>GAAAGVAAWLPFARAAAIGWMPVANCPMPLAPADKNKRQDELIVLNVSGRRFQTWRTTLERYPDTLLGSTEKEFFFNEDTKEYFFDRDPEVFRCVLNFYRTGKLHYPRYECISAYDDELAFYGILPEIIGDCCYEEYKDRKREN[8x];>[8x]EGLEQLEAQTNFTKRELQVLYRGFKNECPSGVVNEDTFKQIYAQFFPHGDASTYAHYLFNAFDTTQTGSVKFEDFVTALSILLRGTVHEKLRWTFNLYDINKDGYINKEEMMDIVKAIYDMMGAYTYPVLAEDTPRQHVDVFFQKMDKNKDGIVTLDEFLESCQE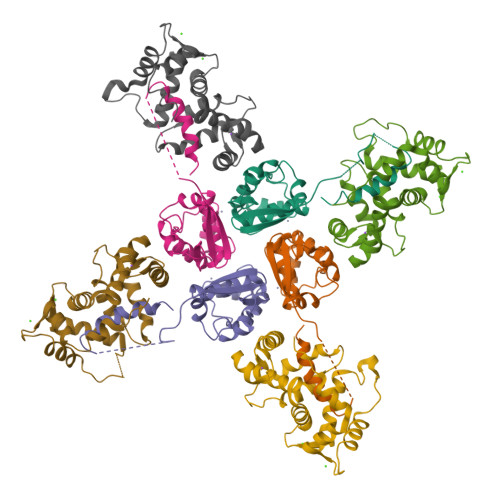DDNIMRSLQLFQNVM> GAHMSGRMTDDKDVLRDVWFGRIPTCFTLYQDEITEREAEPYYLLLPRVSYLTLVTDKVKKHFQKVMRQEDISEIWFEYEGTPLKWHYPIGLLFDLLASSSALPWNITVHFKSFPEKDLLHCPSKDAIEAHFMSCMKEADALKHKSQVINEMQKKDHKQLWMGLQNDRFDQFWAINRKLMEYPAEENGFRYIPFRIYQTTT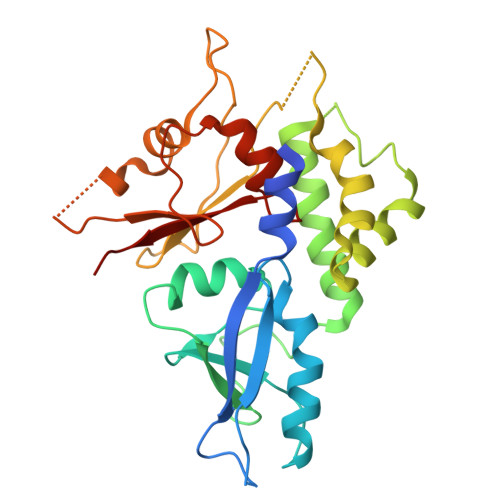ERPFIQKLFRPVAADGQLHTLGDLLKEVCPSAIDPEDGEKKNQVMIHGIEPMLETPLQWLSEHLSYPDNFLHISIIPQPTD> KHYLHDIQKSYLKSRG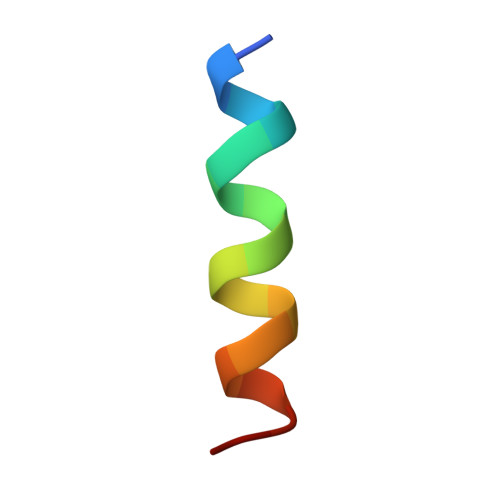N> GEIEFIESSKDAGFPVINTPSKTKLEPSVFHQVFEGNKEPAVLRSGDPRLKANFEEAIFSKYIGNVNTHVDEYMLEAVDHYAGQLATLDISTEPMKLEDAVYGTEGLEALDLTTSAGYPYVALGIKKRDILSKKTKDLTKLKECMDKYGLNLPMVTYVKDELRSIEKVAKGKSRLIEASSLNDSVAMRQTFGNLYKTFHLNPGVVTGSAVGCDPDLFWSKIPVMLDGHLIAFDYSGYDASLSPVWFACLKMILEKLGYTHKETNYIDYLCNSHHLYRDKHYFVRGGMPSGCSGTSIFNSMINNIIIRTLMLKVYKGIDLDQFRM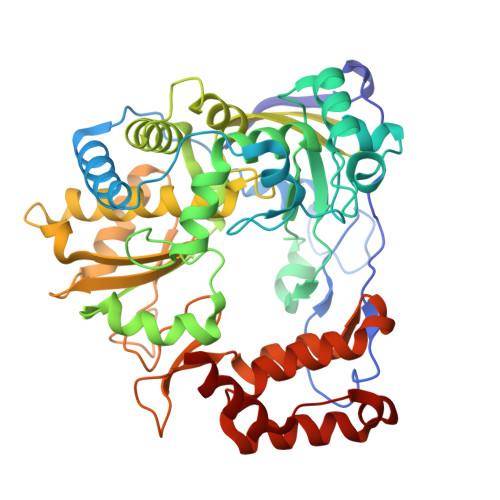IAYGDDVIASYPWPIDASLLAEAGKGYGLIMTPADKGECINEVTWTNVTFLKRYFRADEQYPFLVHPVMPMKDIHESIRWTKDPKNTQDHVRSLCLLAWHNGEHEYEEFIRKIRSVPVGRCLTLPAFSTLRRKWLDSF> SKFLDRFRYFKQKGETFADGHGQLLNTNRDWEDGYRQRWQHDKIVRSTHGVNCTGSCSWKIYVKNGLVTWETQQTDYPRTRPDLPNHEPRGCPRGASYSWYLYSANRLKYPMMRKRLMKMWREAKALHSDPVEAWASIIEDADKAKSFKQARGRGGFVRSSWQEVNELIAASNVYTIKNYGPDRVAGFSPIPAMSMVSYASGARYLSLIGGTCLSFYDWYCDLPPASPQTWGEQTDVPESADWYNSSYIIAWGSNVPQTRTPDAHFFTEVRYKGTKTVAVTPDYAEIAKLCDLWLAPKQGTDAAMALAMGHVMLREFHLDNPSQYFTDYVRRYTDMPMLVMLEERDGYYAAGRMLRAADLVDALGQENNPEWKTVAFNTNGEMVAPNGSIGFRWGEKGKWNLEQRDGKTGEETELQLSLLGSQDEIAEVGFPYFGGDGTEHFNKVELENVLLHKLPVKRLQLADGSTALVTTVYDLTLANYGLERGLNDVNCATSYDDVKAYTPAWAEQITGVSRSQIIRIAREFADNADKTHGRSMIIVGAGLNHWYHLDMNYRGLINMLIFCGCVGQSGGGWAHYVGQEKLRPQTGWQPLAFALDWQRPARHMNSTSYFYNHSSQWRYETVTAEELLSPMADKSRYTGHLIDFNVRAERMGWLPSAPQLGTNPLTIAGEAEKAGMNPVDYTVKSLKEGSIRFAAEQPENGKNHPRNLFIWRSNLLGSSGKGHEFMLKYLLGTEHGIQGKDLGQQGGVKPEEVDWQDNGLEGKLDLVVTLDFRLSSTCLYSDIILPTATWYEKDDMNTSDMHPFIHPLSAAVDPAWEAKSDWEIYKAIAKKFSEVCVGHLGKETDIVTLPIQHDSAAELAQPLDVKDWKKGECDLIPGKTAPHIMVVERDYPATYERFTSIGPLMEKIGNGGKGIAWNTQSEMDLLRKLNYTKAEGPAKGQPMLNTAIDAAEMILTLAPETNGQVAVKAWAALSEFTGRDHTHLALNKEDEKIRFRDIQAQPRKIISSPTWSGLEDEHVSYNAGYTNVHELIPWRTLSGRQQLYQDHQWMRDFGESLLVYRPPIDTRSVKEVIGQKSNGNQEKALNFLTPHQKWGIHSTYSDNLLMLTLGRGGPVVWLSEADAKDLGIADNDWIEVFNSNGALTARAVVSQRVPAGMTMMYHAQERIVNLPGSEITQQRGGIHNSVTRITPKPTHMIGGYAHLAYGFNYYGTVGSNRDEFVVVRKMKNIDWLDGEGNDQVQESVK;> MKIRSQVGMVLNLDKCIGCHTCSVTAKNVWTSREGVEYAWFNNVETKPGQGFPTDWENQEKYKGGWIRKINGKLQPRMGNRAMLLGKIFANPHLPGIDDYYEPFDFDYQNLHTAPEGSKSQPIARPRSLITGERMAKIEKGPNWEDDLGGEFDKLAKDKNFDNIQKAMYSQFENTFMMYLPRLCEHCLNPACVATCPSGAIYKREEDGIVLIDQDKCRGWRMCITGCPYKKIYFNWKSGKSEKCIFCYPRIEAGQPTVCSETCVGRIRYLGVLLYDADAIERAASTENEKDLYQRQLDVFLDPNDPKVIEQAIKDGIPLSV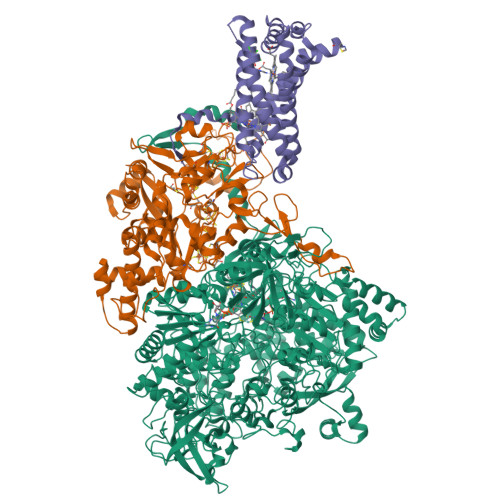IEAAQQSPVYKMAMEWKLALPLHPEYRTLPMVWYVPPLSPIQSAADAGELGSNGILPDVESLRIPVQYLANLLTAGDTKPVLRALKRMLAMRHYKRAETVDGKVDTRALEEVGLTEAQAQEMYRYLAIANYEDRFVVPSSHRELAREAFPEKNGCGFTFGDGCHGSDTKFNLFNSRRIDAIDVTSKTEPHP;> MQFLNMFFFDIYPYIAGAVFLIGSWLRYDYGQYTWRAASSQMLDRKGMNLASNLFHIGILGIFVGHFFGMLTPHWMYEAWLPIEVKQKMAMFAGGASGVLCLIGGVLLLKRRLFSPRVRATTTGADILILSLLVIQCALGLLTIPFSAQHMDGSEMMKLVGWAQSVVTFHGGASQHLDGVAFIFRLHLVLGMTLFLLFPFSRLIHIWSVPVEYLTRKYQLVRARH> GPPSGKTYMGWWGHMGGPKQKGITSYAVSPYAQKPLQGIFHNAVFNSFRRFKSQFLYVLIPAGIYWYWWKNGNEYNE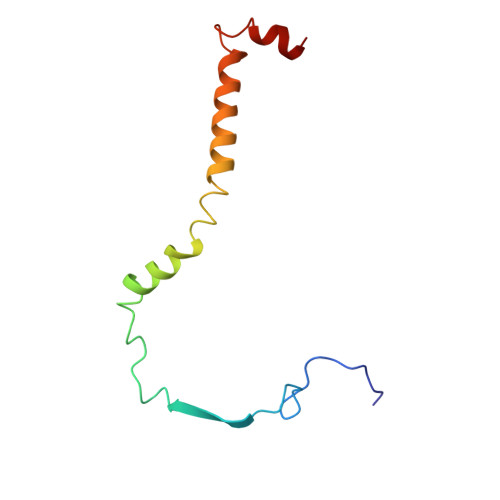FLYSKAGREELERVNV> GSEDLPHHDEKTWNVGSSNRNKAENLLRGKRDGTFLVRESSKQGCYACSVVVDGEVKHC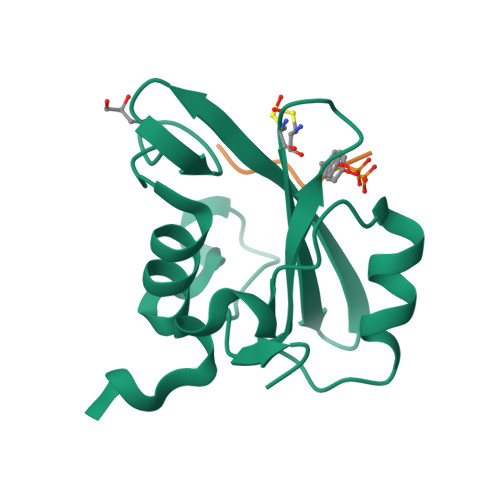VINKTATGYGFAEPYNLYSSLKELVLHYQHTSLVQHNDSLNVTLAYPVYA;> SDYMNMTP> MAHHHHHHMGSRISKEAAPVTFKNGKPTVKGTKTYP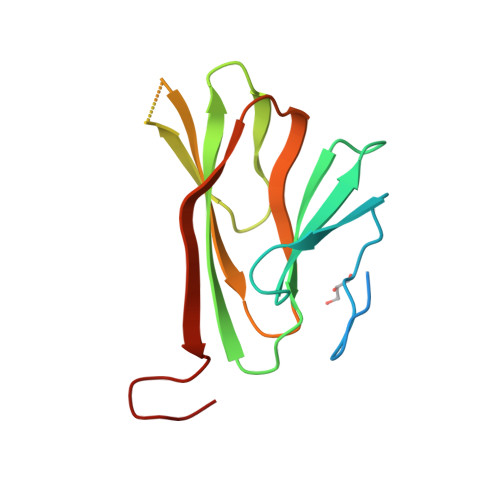MFSNILYRIADTEARRWAFYNDSKELIIHVAVLFDYDSQIVPLGDTTAFRIDDPDEGNEDDFGKYLCEVDVRPLETQMFVEGSVTGWRVDTLEARTAEDERGYRL> SDLTVSLEEASRLESENVKRLRQEKRLSLIVDLDQTIIHATVDPTVGEWMSDPGNVNYDVLRDVRSFNLQEGPSGYTSCYYIKFRPGLAQFLQKISELYEL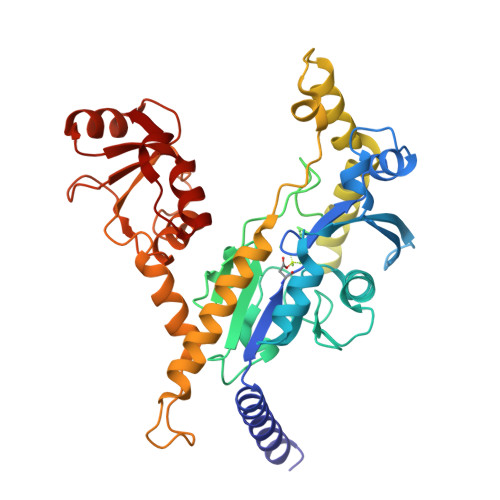HIYTMGTKAYAKEVAKIIDPTGKLFQDRVLSRDDSGSLAQKSLRRLFPCDTSMVVVIDDRGDVWDWNPNLIKVVPYEFFVGIGDINSNFLAKSTPLPEQEQLIPLEIPKDEPDSVDEINEENEETPEYDSSNSSYAQDSSTIPEKTLLKDTFLQNREALEEQNKERVTALELQKSERPLAKQQNALLEDEGKPTPSHTLLHNRDHELERLEKVLKDIHAVYYEEENDISSRSGNHKHANVGLIIPKMKQKVLKGCRLLFSGVIPLGVDVLSSDIAKWAMSFGAEVVLDFSVPPTHLIAAKIRTEKVKKAVSMGNIKVVKLNWLTESLSQWKRLPESDYLLY Two enzymes, peptidylglycine α-hydroxylating monooxygenase (PHM; EC 1.14.17.3) and peptidyl-α-hydroxyglycine α-amidating lyase (PAL; EC 4.3.2.5) working sequentially are the only proteins known to catalyze this reaction. PHM, a two Cu enzyme, catalyzes the stereospecific hydroxylation of the glycine Cα of peptidylglycine substrates. The two copper atoms in PHM, CuH, and CuM (located in the N- and C-subdomains, respectively), each use a single reducing equivalent from ascorbate to catalyze the reduction of molecular oxygen for the hydroxylation of the Cα of glycine at the carboxy-terminus of the peptide substrate. Crystallographic data on apo wild-type PHM and on several crystal forms of three CuH mutants (H107A, H108A, and H172A) presented here show that the copper ions are required not only for the catalytic steps but also for substrate binding and for locking the overall conformation of PHM in a configuration that is catalytically active.

As a step toward this goal, we have determined the structures of the apo-enzyme and three His variants at the H-center-H107A, H108A, and H172A, all without the addition to Cu2+ in the crystallization media. All of the PHM structures published to date contain two copper ions. As expected, there was no density for either of the two coppers—CuH or CuM. The final R-values are Rwork = 20.9% and Rfree = 27.3%. While loss of both coppers in the structure of apo PHM has no significant effect on the conformation of the molecule, mutations that cause loss of copper from a single site appear to have significant effects.

> NECLGTIGPVTPLDASDFALDIRMPGVTPKESDTYFCMSMRLPVDEEAFVIDFKPRASMDTVHHMLLFGCNMPSSTGSYWFCDEGTCTDKANILYAWARNAPPTRLPKGVGFRVGGETGSKYFVLQVHYGDISAFRDNHKDCSGVSVHLTRVPQPLIAGMYLMMSVDTVIPPGEKVVNADISCQYKMYPMHVFAYRVHTHHLGKVVSGYRVRNGQWTLIGRQNPQLPQAFYPVEHPVDVTFGDILAARCVFTGEGRTEATHIGGTSSDEMCNLYIMYYMEAKYALSFMTCTKNVAPDMFRTIPAEANIPIPV> GSKESCPSVSIPSSDEHREKKKRFTVYKVLVSVGRSEWFVFRRYAEFDKLYNTLK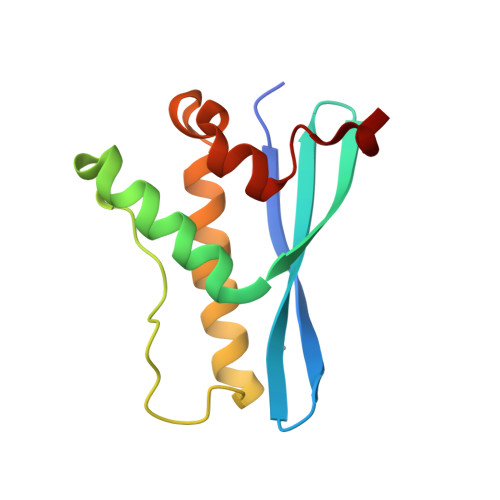KQFPAMALKIPAKRIFGDNFDPDFIKQRRAGLNEFIQNLVRYPELYNHPDVRAFLQMDSPKHQ3,3',3''-phosphoryltripropanoic 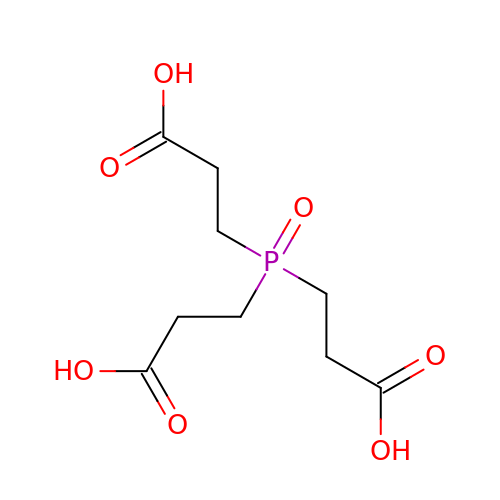acid | C9 H15 O7 P | XJGZCDJZBUBTKW-UHFFFAOYSA-N> MFQRTCTPRLLACTSALLKRSGKPSDLPDYKQV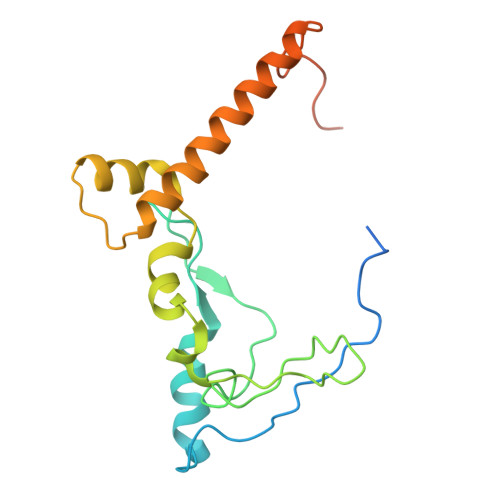YLPYDTAPTKTELDRERRKFMHAYSGRMEHRKMVEVKDVPQNMYTYGKEGMSIPISIFKDQADPVIGPEWTYPGIFENKIVAQHWYMEELFDREKSNTFESPWQRQVLDNQVKRRLGKVAWRMSMLNIKTIDIFHKERGASKRPGAGDTKAPATPAGKK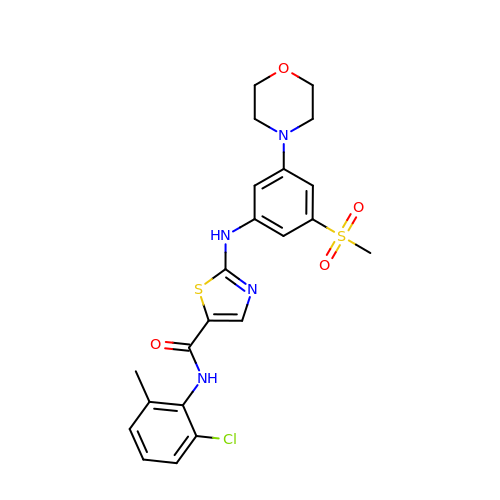~{N}-(2-chloranyl-6-methyl-phenyl)-2-[(3-methylsulfonyl-5-morpholin-4-yl-phenyl)amino]-1,3-thiazole-5-carboxamide | C22 H23 Cl N4 O4 S2 | JWVBEFCCTKVFPM-UHFFFAOYSA-N2-{3,5-dimethyl-4-[2-(pyrrolidin-1-yl)ethoxy]phenyl}-5,7-dimethoxyquinazolin-4(3H)-one | C24 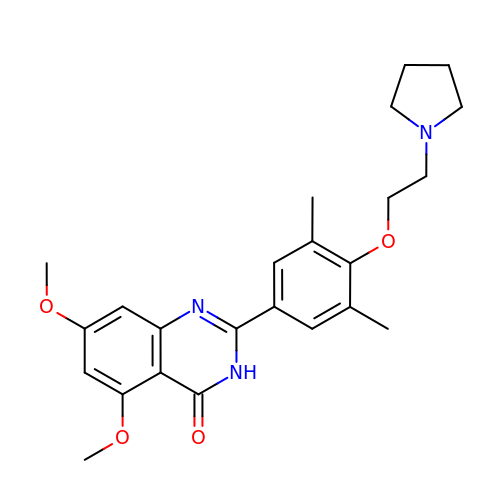H29 N3 O4 | PQZDYFRDRHRZGF-UHFFFAOYSA-N>MAHHHHHHRK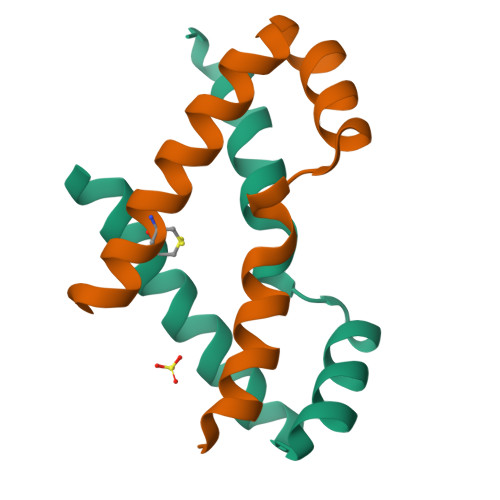KTKEQIAHLKASFLQSQFPDDAEVYRLIEVTGLARSEIKKWFSDHRYRCQRGIVHI[2x]>MGGSGSRLSKELLAEYQDLTFLTKQEILLAHRRFCELLPQEQRSVESSLRAQVPFEQILSLPELKANPFKERICRVFSTSPA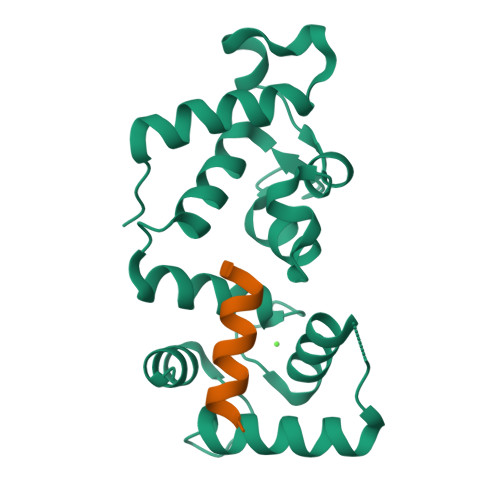KDSLSFEDFLDLLSVFSDTATPDIKSHYAFRIFDFDDDGTLNREDLSRLVNCLTGEGEDTRLSASEMKQLIDNILEESDIDRDGTINLSEFQHVISRSPDFASSFKIVL[4x];>DGGSFWYRAMKALYG[4x]> GDDVMTKEEQIFLLHRAQAQCEKRLKEVLQRPAGRPCLPEWDHILCWPLGAPGEVVAVPCPDYIYDFNHKGHAYRRCDR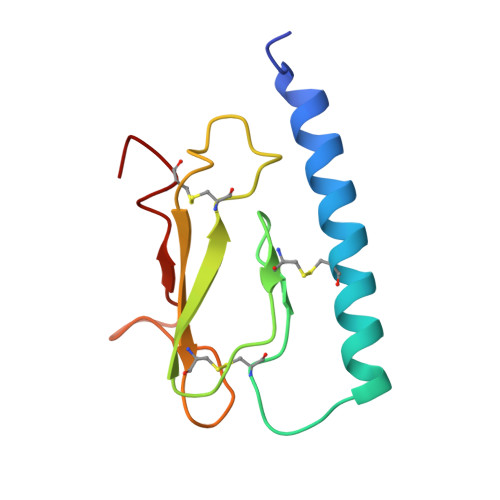NGSWELVPGHNRTWANYSECVKFL>[2x]GVNPRGLGPLQIWQTDFTLEPRMAPRSWLAVTVDTASSAIVVTQHGRVTSVAVQHHWATAIAVLGRPKAIKTDNGS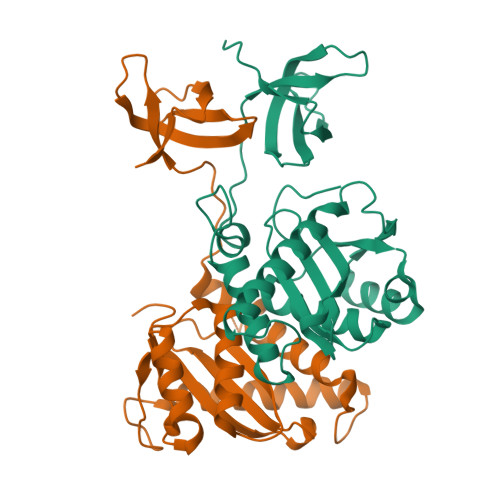CFTSKSTREWLARWGIAHTTGIPGNSQGQAMVERANRLLKDRIRVLAEGDGFMKRIPTSKQGELLAKAMYALNHKERGENTKTPIQKHWRPTVLTEGPPVKIRIETGEWEKGWNVLVWGRGYAAVKNRDTDKVIWVPSRKVKPDITQKDEVTKKDEASPLFA> MYGSKTFIKYVSGIPDYFKQSFPEGF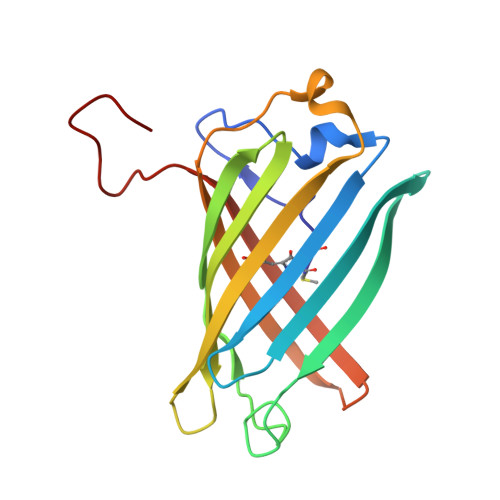TWERTTTYEDGGFLTAHQDTSLDGDCLVYKVKILGNNFPADGPVMQNKAGRWEPGTEIVYEVDGVLRGQSLMALKCPGGRHLTCHLHTTYRSKKPASALKMPGFHFEDHRIEIMEEVEKGKCYKQYEAAVGRYCDAAPSKLGHN>GSHM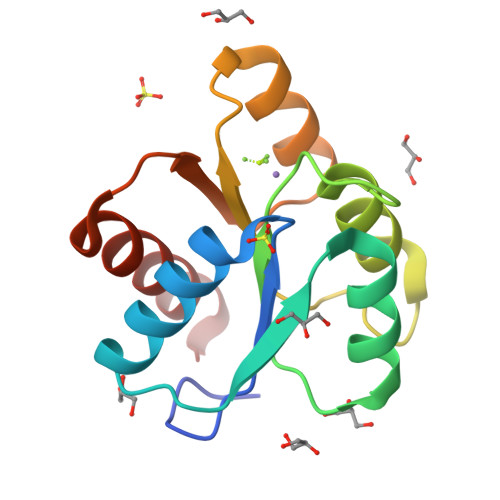ADKELKFLVVDDFSTMRRIVRNLLKELGFNNVEEAEDGVDALNKLQAGGYGFVISDWDMPNMDGLELLKTIRADGAMSALPVLMVTAYAKKENIIAAAQAGASGYVVKPFTAATLEEKLNKIFEKLGM[2x]> SLSEQALNHEKLMRAIVKNLADTPMVLKGETALYLGYGLNRFSEDLDFDCHKKINLLGRVKSAIPNGIILNDIHIKKDTDSVGRYMVRYATKDNKEEQTLKLEISYR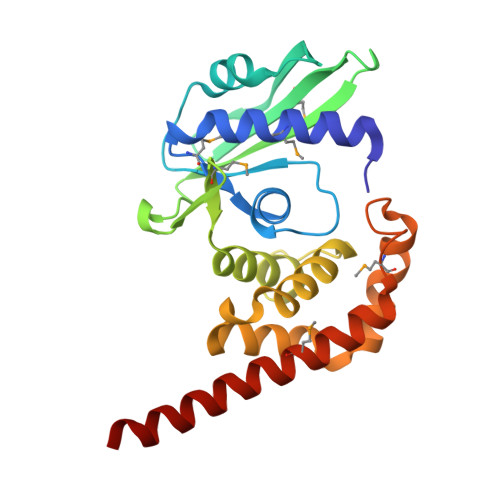DAPKESEVNVIEGMRIAKIERIIDNKLCACFDGEHTRTKARDLFDLHFLAKHYEEHFNLDLASRLKDFSKDPDKLVSDYLVDVKLDALLNQIMDLEETALELGVMAQLIHKKLEKQSHSLNALQE> SNAMPSKLSRLELLPAVDVRDGQAVRLVHGESGTETSYGSPLEAALSWQRAGAEWLHLVDLDAAFGTGDNRELVRQVTEAMDIKVELSGGIRDDASLAAALATGCTRVNLGTAALE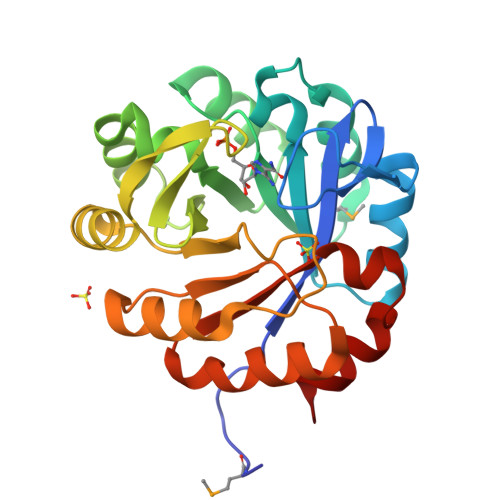SPEWVAKVIAEHGDRIAVGLDVRGTTLKGRGWTSEGGDLYEALERLDKEGCARYVVTDIAKDGTLQGPNLELLRNVCAATDRPVVASGGVSSLDDLRAIAELVPLGVEGSIVGKALYAKAFTLEEALEAVAQ>MKNIGWMLRQRATVSPRLQAYVEPSTDVRMTYAQM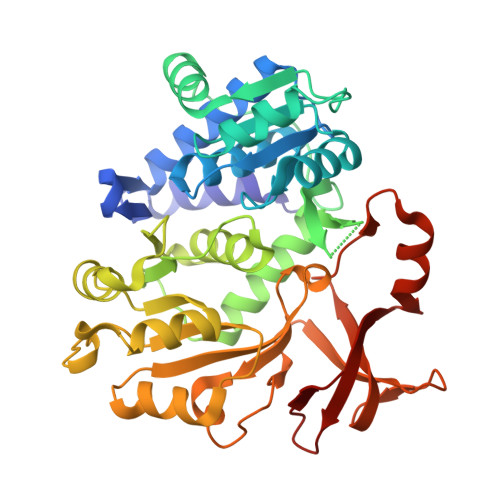NALANRCADVLTALGIAKGDRVALLMPNSVEFCCLFYGAAKLGAVAVPINTRLAAPEVSFILSDSGSKVVIYGAPSAPVIDAIRAQADPPGTVTDWIGADSLAERLRSAAADEPAVECGGDDNLFIMYTSGTTGHPKGVVHTHESVHSAASSWASTIDVRYRDRLLLPLPMFHVAALTTVIFSAMRGVTLISMPQFDATKVWSLIVEERVCIGGAVPAILNFMRQVPEFAELDAPDFRYFITGGAPMPEALIKIYAAKNIEVVQGYALTESCGGGTLLLSEDALRKAGSAGRATMFTDVAVRGDDGVIREHGEGEVVIKSDILLKEYWNRPEATRDAFDNGWFRTGDIGEIDDEGYLYIKD[2x]>MAEAASCARKGTKYAEGTQPFTVLIEGNIGSGKTTYLNHFEKYKNDICLLTDPVEKWRNVNGVNLLELMYKDPKKWAMPFQSYVTLTMLQSHTAPTNKKLKIMERSIFSARYCFVENMRRNGSLEQGMYNTLEEWYKFIEESIHVQADLIIYLRTSPEVAYERIRQRA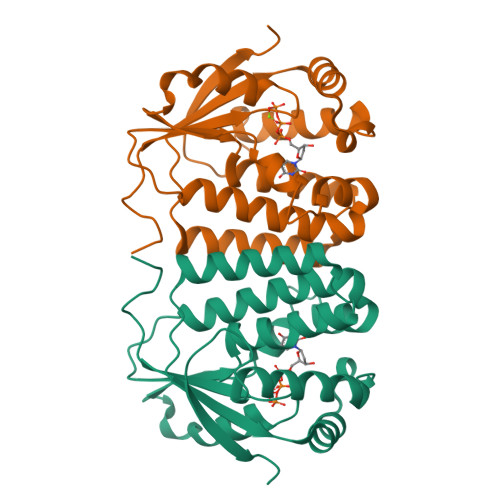RSEESCVPLKYLQELHELHEDWLIHQRRPQSCKVLVLDADLNLENIGTEYQRSESSIFDAIS[2x]>MFDKHTHTLIAQRLDQAEKQREQIRAISLDYPEITIEDAYAVQREWVRLKIAEGRTLKGHKIGLTSKAMQASSQISEPDYGALLDDMFFHDGSDIPTDRFIVPRIEVELAFVLAKPLRGPNCTLFDVYNATDYVIPALELIDARCHNIDPETQRPRKVFDTISDNAANAGVILGGRPIKPDEL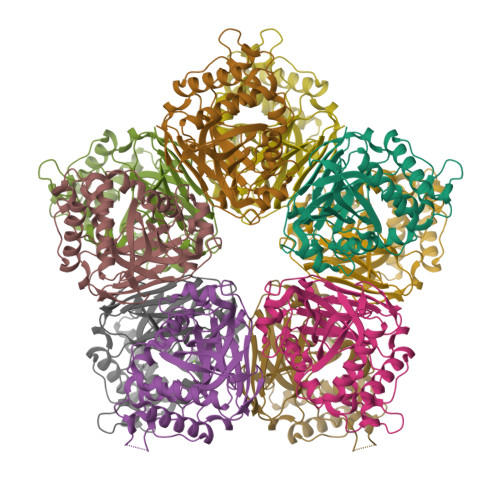DLRWISALMYRNGVIEETGVAAGVLNHPANGVAWLANKLAPYDVQLEAGQIILGGSFTRPVPARKGDTFHVDYGNMGSISCRFV[5x]Three salutaridine/menthone reductase like subfamilies of short‐chain dehydrogenases/reductases (SDRs)2 from Mentha piperita were identified, namely (−)‐menthone:(−)‐menthol reductase (MMR), (−)‐menthone:(+)‐neomenthol reductase (MNMR), and isopiperitenone reductase (IPR).1a,1b MMR and MNMR catalyze the ketoreduction of (−)‐menthone 1 a to (1R,2S,5R)‐menthol 2 a and (1S,2S,5R)‐neomenthol 2 b, respectively.1a Additionally, they act on isomenthone 1 b to produce (1R,2R,5R)‐neoisomenthol 2 c and (1R,2S,5S)‐isomenthol 2 d, respectively. Interestingly, the three Mentha SDRs have high protein‐sequence identities (63–68 %), so we performed comparative studies of MMR, MNMR, and IPR, to pinpoint the determinants of ketoreductase vs. ene‐reductase activity within SDRs. A key difference in the sequences between the ketoreductases and IPR was a substitution of the highly conserved catalytic Tyr residue for Glu (238 in IPR). We determined crystal structures of both MNMR and IPR, the latter in combination with NADP+, alkene 3 a, and β‐cyclocitral (non‐substrate).

The IPR–β‐cyclocitral co‐crystal structure shows the ligand binds in a non‐active conformation compared to 3 a binding. No other major changes in residue positions were observed in the co‐crystal structures.

> GAMAEVQRYALVTGANKGIGFEICRQLAEKGIIVILTSRNEKRGLEARQKLLKELNVSENRLVFHQLDVTDLASVAAVAVFIKSKFGKLDILVNNAGVSGVEMVGDVSVFNEYIEADFKALQALEAGAKEEPPFKPKANGEMIEKFEGAKDCVVTNYYGPKRLTQALIPLLQLSPSPRIVNVSSSFGSLLLLWNEWAKGVLGDEDRLTEERVDEVVEVFLKDIKEGKLEESQWPPHFAAERVSKAALNAYTKIAAKKYPSFRINAICPGYAKTDITFHAGPLSVAEAAQVPVKLALLPDGGPSGCFFPRDKALALYLE>[4x]MNPAAEAEFNILLATDSYKVTHYKQYPPNTSKVYSYFECREKKTENSKLRKVKYEETVFYGLQYILNKYLKGKVVTKEKIQEAKDVYKEHFQDDVFNEKGWNYILEKYDGHLPIEIKAVPEGFVIPRGNVLFTVENTDPECYWLTNWIETILVQSWYPITVATNSREQKKILAKY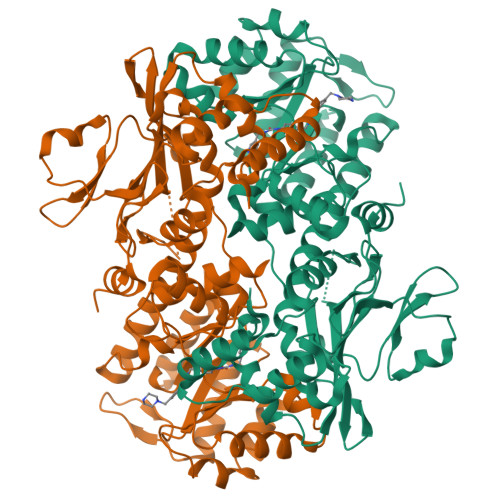LLETSGNLDGLEYKLHDFGYRGVSSQETAGIGASAHLVNFKGTDTVAGLALIKKYYGTKDPVPGYSVPAAEHSTITAWGKDHEKDAFEHIVTQFSSVPVSVVSDSYDIYNACEKIWGEDLRHLIVSRSTQAPLIIRPDSGNPLDTVLKVLEILGKKFPVTENSKGYKLLPPYLRVIQGDGVDINTLQEIVEGMKQKMWSIENIAFGSGGGLLQKLTRDLLNCSFKCSYVVTNGLGINVFKDPVADPNKRSKKGRLSLHRTPAGNFVTLEEGKGDLEEYGQDLLHTVFKNGKVTKSYSFDEIRKNAQLNIELEAAHHLEHHHHHHHH>[4x]AYSNTYQEFTNIDQAKAWGNAQYKKYGLSKSEKEAIVSYTKSASEINGKLRQNKGVINGFPSNLIKQVELLDKSFNKMKTPENIMLFRGDDPAYLGTEFQNTLLNSNGTINKTAFEKAKA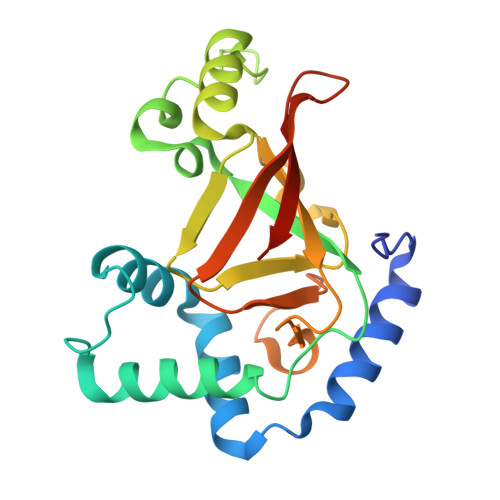KFLNKDRLEYGYISTSLMNVSQFAGRPIITKFKVAKGSKAGYIDPISAFAGQLEMLLPRHSTYHIDDMRLSSDGKQIIITATMMGTAINPK> QAQITGRPEWIWLALGTALMGLGTLYFLVKGMGVSDPDAKKFYAITTLAPAIAFTMYLSMLLGYGLTMVPFGGEQNPIYWARYADWLFTTPLLLLDLALLVDADQGTILALVGADGIMIGTGLVGALTKVYSYRFVWWAISTAAMLYILYVLFFGFTSKAESMRPEVASTFKVLRNVTVVLWSAYPVVWLIGSEGAGIVPLNIETLLFMVLDVS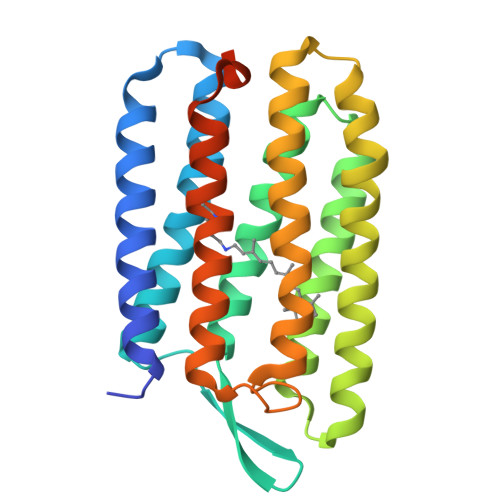AKVGFGLILLRSRAIFGEAEAPEPSAGDGAAATSD The betaproteobacteria Burkholderia pseudomallei and Burkholderia mallei, causative agents of melioidosis and glanders, respectively, encode the TssM effector, the only known bacterial DUB belonging to the USP class. By solving the crystal structures of isolated TssM and its complex with ubiquitin, we found that TssM lacks the entire “Fingers” subdomain of the USP fold. Instead, the TssM family has evolved the functionally analog “Littlefinger” loop, which is located towards the end of the USP domain and recognizes different ubiquitin interfaces than those used by USPs. The structures revealed the presence of an N-terminal immunoglobulin-fold domain, which is able to form a strand-exchange dimer and might mediate TssM localization to the bacterial surface.

To better understand the evolutionary position of TssM within the USP family and its possible relationship with the Josephin family, we solved the crystal structure of TssM193–490 to a resolution of 3.15 Å. This construct comprises the portion of TssM predicted to be structured, and upon crystallization revealed the presence of two globular folds: an N-terminal immunoglobulin-like domain, followed by the catalytic DUB domain. The asymmetric unit contained two TssM molecules forming a possible dimer with a contact surface formed by the Ig-like domains, with some contributions by the catalytic domain. A single β-strand formed by the first eight residues of the Ig-like domain is swapped between the two adjacent dimers. The two chains are almost completely resolved, with the exception of residues 193 (chain B), 394, and 395 missing from both monomers, and residues 476–480 being disordered in chain B. Both chains have identical conformations and can be superimposed with an RMSD of 0.63 Å for 3,221 atoms. The DUB domain assumed a papain-like fold with an active site triad formed by Cys-308, His-442, and Asp-457. When matching the entire USP folds of TssM and USP7, the resulting RMSD of 5.4 Å is unusually high. This discrepancy is owed to the fact that the TssM structure lacks the entire Fingers subdomain, which is in accordance with the major deletion observed in the multiple sequence alignment within the respective region. In TssM, the entire deleted region is replaced by the short helix α6 flanked by flexible loops, which appear neither related to other USP domains, nor do they structurally correspond to canonical USP elements. Whereas the Ub-PA–bound structure contains two individual barely interacting TssM ∼ Ub-PA complexes, the apo structure shows the Ig-like domains in a strand-swapped dimer, in which the first β-strand of each Ig-like domain folds with the remainder of the adjacent molecule. The β-strand swap observed in the apo-structure does not appear to stabilize a TssM dimer in solution and might be a crystallization artifact.

>[2x]GPPAVVATRVPPTHAALRRPTIELEFDRAIEPGSVPHIVLRADDGTSVAVGPLSWLSDRRIAFAPRKPLKSNSRYEIMVPAGIRSTTGERSTHPLTSSFDTAPVTPPRGLPNLDGASCFINTALQLAVHSSALDDILSNEAVPPAVRTLLEDYDAASADALDAQLAAAVAALRATPEVPDSGPGQTLEVMQALRMPLYDTSSANNAKNNADAIRHAPPNTKAFFLNSYPPLSYADLPNHDRLVAFDYSTGGHYVAYVKRDGIWYRIDDAQVSAVNEQDLLALPAFNPANGSVSIEIAIYR> MRRTVVQRVAPWVPPPRHDIKVTMPPPPGGEVGGRFGVSQGYSDRLARTPYWKRMALSTYKLRMMENATRYPMSEHRPGEYDIRYLPTPYPCTIRNRPLLEVGEPRQIPSIRIPVIFLVNLFDEAKGCWFGRRYETVYVERQFMREELM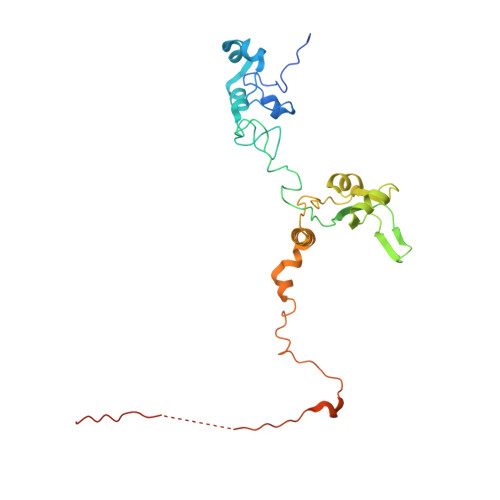PQRYAIYATPEAYKLLGLPVVNHHTHEEIPKTPREYEKLLERQRYDEERWKYTIEYLFRKYEDGPPELLDRPEDGWDGSEEIALSSVAGAGRDGVVSQRXXXXXXXXXXKIKLF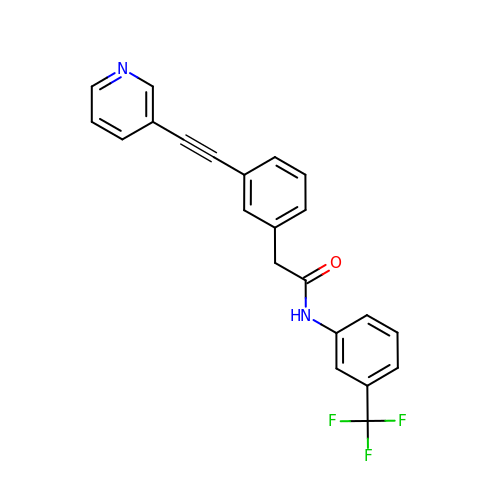2-{3-[(pyridin-3-yl)ethynyl]phenyl}-N-[3-(trifluoromethyl)phenyl]acetamide | C22 H15 F3 N2 O | NGGVWQHQHPAORG-UHFFFAOYSA-N>GAMGRILFLTTFMSKGNKVVRYLESLHHEVVICQEKVHAQSANLQEIDWIVSYAYGYILDKEIVSRFRGRIINLHPSLLPWNKGRDPVFWSVWDETPKGVTIHLIDEHVDTGDILVQEEIAFADEDTLLDCYNKANQAIEELFIREWENIVHGRIAPYRQTAGGTLHFKADRDFYKNLNMTTVRELLALKRLCAEPKRGEKPIDKTFHQLFEQQVEMTPDHVAVVDRGQSLTYKQLNERANQLAHHLRGKGVKPDDQVAIMLDKSLDMIVSILAVMKAGGAYVPIDPDYPGERIAYMLADSSAAILLTNALHEEKANGACDIIDVHDPDSYSENTNNLPHVNRPDDLVYVMYTSGSTGLAKGVMIEHHNLVNFCEWYRPYFGVTPADKALVYSSFSFDGSALDIFTHLLAGAALHIVPSERKYDLDALNDYCNQEGITISYLPTGAAEQFMQMDNQSFRVVITGGDVLKKIERNGTYKLYNGYGPTECTIMVTMFEVDKPYANIPIGKPIDRTRILILDEALALQPIGVAGELFIVGEGLGRGYLNRPELTAEKFIVHPQTGERMYRTGDRARFLPDGNIEFLGRLDNLVKIRGYRIEPGEIEPFLMNHPLIELTTVLAKEQADGRKYLVGYYVAPEEIPHGELREWLGNDLPDYMIPTYFVHMKAFPLTANGKVDRRALPDVQADAELLGEDYVAPTDELEQQLAQVWSHVLGIPQMGIDDHFLERGGDSIKVMQLIHQLKNIGLSLRYDQLFTHPTIRQLKRLLTEQKQVSLEPLRELDEQAEYETSAVEKRMYIIQQQDVESIAYNVVYTINFPLTVDTEQIRVALEQLVLRHEGLRSTYHMRGDEIVKRIVPRAELSFVRQTGEEESVQSLLAEQIKPFDLAKAPLLRAGVIETADKKVLWFDSHHILLDGLSKSILARELQALLGQQVLSPVEKTYKSFARWQNEWFASDEYEQQIAYWKTLLQGELPAVQLPTKKRPPQLTFDGAIQMYRVNPEITRKLKATAAKHDLTLYMLMLTIVSIWLSKMNSDSNQVILGTVTDGRQHPDTRELLGMFVNTLPLLLSIDHEESFLHNLQQVKAKLLPALQNQYVPF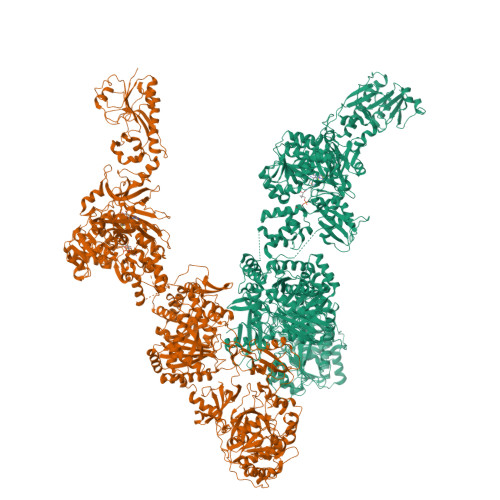DKILEAARVKREGNRHPLFDVMFMMQGAPETELESNMHHINAGISKFDLTLEVLERENGLNIVFEYNTHLFDEGMILRMVAQFEHLLLQAVHGLDQQVKRFELVTEDEKRDLFLRVNDTAKAYPNKLIMSMLEDWAAATPDKTALVFREQRVTYRELNERVNQLAHTLREKGVQPDDLVMLMAERSVEMMVAIFAVLKAGGAYLPIDPHSPAERIAYIFADSGAKLVLAQSPFVEKASMAEVVLDLNSASSYAADTSNPPLVNQPGDLVYVMYTSGSTGKPKGVMIEHGALLNVLHGMQDEYPLLQDDAFLLKTTYIFDISVAEIFGWVPGRGKLVILEPEAEKNPKAIWQAVVGAGITHINFVPSMLIPFVEYLEGRTEANRLRYILACGEAMPDELVPKVYEVLPEVKLENIYGPTEATIYASRYSLAKGSQESPVPIGKPLPNYRMYIINRHGQLQPIGVPGELCIAGASLARGYLNNPALTEEKFTPHPLEKGERIYRTGDLARYREDGNIEYLGRMDHQVKIRGYRIELDEIRSKLIQEETIQDAVVVARNDQNGQAYLCAYLLSEQEWTVGQLRELLRRELPEYMIPAHFVLLKQFPLTANGKLDRKALPEPDGSVAAAENLYFQ[2x]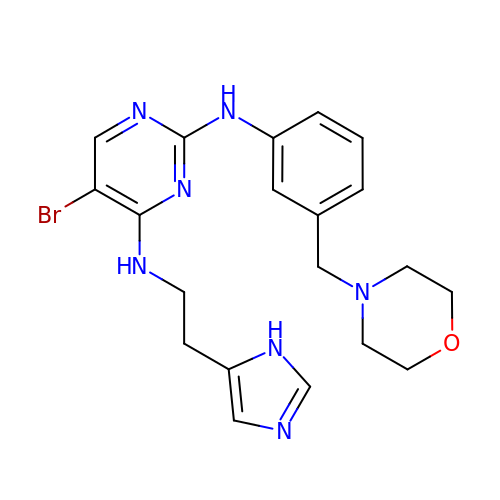5-Bromo-4-N-[2-(1H-imidazol-5-yl)ethyl]-2-N-[3-(morpholin-4-ylmethyl)phenyl]pyrimidine-2,4-diamine | C20 H24 Br N7 O | IOYFYUOBKSQTFF-UHFFFAOYSA-N>DYKDDDDKGSGSGIAELPPKVSVFVPPRDGFFGNPRKSKLICQATGFSPRQIQVSWLREGKQVGSGVTTDQVQAEAKESGPTTYKVTSTLTIKESDWLSQSMFTCRVDHRGLTFQQNASSMCVPDQDTAIRVFAIPPSFASIFLTKSTKLTCLVTDLTTYDSVTISWTRQNGEAVKTHTNISESHPNATFSAVGEASICEDDWNSGERFTCTVTHTDLPSPLKQTISRPKGVALHRPDVYLLPPAREQLNLRESATITCLVTGFSPADVFVQWMQRGQPLSPEKYVTSAPMPEPQAPGRYFAHSILTVSEEEWNTGETYTCVVAHEALPNRVTERTVDKSTGKPTLYNVSLVMSDTAGTCY[4x];> MKNHLLFWGVLAVFIKAVHVKAQEDERIVLVDNKCKCARITSRIIRSSEDPNEDIVERNIRIIVPLNNRENISDPTSPLRTRFVYHLSDLCKKCDPTEVELDNQIVTATQSNICDEDSATETCYTYDRNKCYTAVVPLVYGGETKMVETALTPDACYPDEQKLISEEDL;> SPSGVRLVGGLHRCEGRVEVEQKGQWGTVCDDGWDIKDVAVLCRELGCGAASGTPSGILYEPPAEKEQKVLIQSVSCTGTEDTLAQCEQEEVYDCSHDEDAGASCENPESSFSPVPEGVRLADGPGHCKGRVEVKHQNQWYTVCQTGWSLRAAKVVCRQLGCGRAVLTQKRCNKHAYGRKPIWLSQMSCSGREATLQDCPSGPWGKNTCNHDEDTWVECEDPFDLRLVGGDNLCSGRLEVLHKGVWGSVCDDNWGEKEDQVVCKQLGCGKSLSPSFRDRKCYGPGVGRIWLDNVRCSGEEQSLEQCQHRFWGFHDCTHQEDVAVICSG

Apoptosis inhibitor of macrophage (AIM/CD5L) is a soluble protein belonging to the scavenger receptor cysteine-rich (SRCR) superfamily that contributes to prevention of a wide range of diseases associated with infection, inflammation, and cancer. AIM forms complexes with IgM pentamers which helps maintain high-levels of circulating AIM in serum for subsequent activation on release from the complex. Here we apply cryogenic electron microscopy imaging (cryo-EM) to show how interfaces on both of AIM’s C-terminal SRCR domains interact with the Fcμ constant region and J chain components of the IgM core. The human Fcμ/J/AIM complex shows the binding of tandem AIM SRCR domains to IgM leading to sequestration and stabilisation of AIM.

AIM recognises IgM at both Fcμ and J chain. The total buried surface area (BSA) between AIM and IgM is 994 Å2, with 652 Å2 between AIM and J chain and 342 Å2 between AIM and subunit Fcμ5. The unpaired cysteine residue C191 in SRCR2AIM forms a disulfide bond with C414 in Cμ3-5B, which aligns with the fact that AIM does not dissociate from IgM during SDS–polyacrylamide gel electrophoresis in non-reducing conditions. This disulfide bond is crucial, as the C191S mutant completely abolished the binding between IgM and AIM, as previously shown. In addition, K173 and R183 in SRCR2 form two salt bridges with β-hairpin 2 of J chain at E77 and E75. SRCR3AIM sits between β-hairpin 2 and β-hairpin 3 of J chain and interacts with both loops. F329 and F332 on SRCR3 pack against P96 in β-hairpin 2 of J chain through a van der Waals contact, plus a salt bridge between D72 and R328.Biological evaluation revealed that apoxidoles define a new potent type IV inhibitor chemotype of indoleamine 2,3‐dioxygenase 1 (IDO1), a heme‐containing enzyme considered a target for the treatment of neurodegeneration, autoimmunity and cancer. The three tryptophan‐catabolizing enzymes indoleamine 2,3‐dioxygenase 1 and 2 (IDO1 and IDO2) and tryptophan 2,3‐dioxygenase (TDO) catalyze the first and rate‐limiting step of the Kyn pathway. The IDO1 active site consists of four sub‐pockets A to D, of which pockets A, B and C are normally separated from pocket D by the cofactor heme. In contrast to inhibitor types I–III, type IV inhibitors do not coordinate to the heme in the IDO1 active site, but target IDO1 exclusively in its heme‐free form.

A co‐crystal structure of apoxidole‐1 with apo‐IDO1 was solved to determine the binding mode of the compound. The crystal structure revealed that apoxidole‐1 binds to pockets A and D, occupying the heme‐binding site spanning both pockets. Residues 360–383 belonging to the JK‐loop are not resolved in this structure, thus indicating a flexible structural element. Residue Phe270 adopts a conformation similar to structures of holo‐IDO1 without a proximal pocket D ligand. Consequently, pocket D is in an open conformation and allows for solvent exchange between helices E and F. Furthermore, Leu384 on the N‐terminal side of helix K points into the free heme‐binding pocket as typically observed for structures of apo‐IDO1. The ligand is framed by the hydrophobic amino acids Tyr126, Phe163, Phe214, Phe226, Leu234, Phe270, and Leu342 and is additionally stabilized by polar interactions between the carbonyl oxygen of the ethyl ester of apoxidole‐1 and His346 which is normally coordinated to the proximal site of heme in holo‐IDO1. Similar to other co‐crystal structures, we observed unexplained electron density in close proximity to the tosyl in pocket D. In contrast to the ligand core, the tosyl appendage of apoxidole‐1 is flexible. Hence, we modelled two different conformations of the ligand with the tosyl pointing in different directions (green and cyan sticks). Considering this and the large free space in pocket D, this part of the ligand structure could be further derivatized to achieve higher occupancies, possibly improving the affinity to IDO1. Apoxidole‐1 dose‐dependently reduced the Soret peak, proving that compound binding to IDO1 releases heme.

> GPLGSGIQMENSWTISKEYHIDEEVGFALPNPQENLPDFYNDWMFIAKHLPDLIESGQLRERVEKLNMLSIDHLTDHKSQRLARLVLGCITMAYVWGKGHGDVRKVLPRNIAVPYCQLSKKLELPPILVYADCVLANWKKKDPNKPLTYENMDVLFSFRDGDCSKGFFLVSLLVEIAAASAIKVIPTVFKAMQMQERDTLLKALLEIASCLEKALQVFHQIHDHVNPKAFFSVLRIYLSGWKGNPQLSDGLVYEGFWEDPKEFAGGSAGQSSVFQCFDVLLGIQQTAGGGHAAQFLQDMRRYMPPAHRNFLCSLESNPSVREFVLSKGDAGLREAYDACVKALVSLRSYHLQIVTKYILIPASQQPKENKTSEDPSKLEAKGTGGTDLMNFLKTVRSTTEKSLL> DSSDEASVSPIADNEREAVTLLLGYLEDKDQLDFYSGGPLKALTTLVYSDNLNLQRSAALAFAEITEKYVRQVSREVLEPILILLQSQDPQIQVAACAALGNLAVNNENKLLIVEMGGLEPLINQMMGDNVEVQCNAVGCITNLATRDDNKHKIATSGALIPLTKLAKSKHIRVQRNATGALLNMTHSEENRKELVNAGAVPVLVSLLSSTDPDVQYYCTTALSNIAVDEANRKKLAQTEPRLVSKLVSLMDSPSSRVKCQATLALRNLASDTSYQLEIVR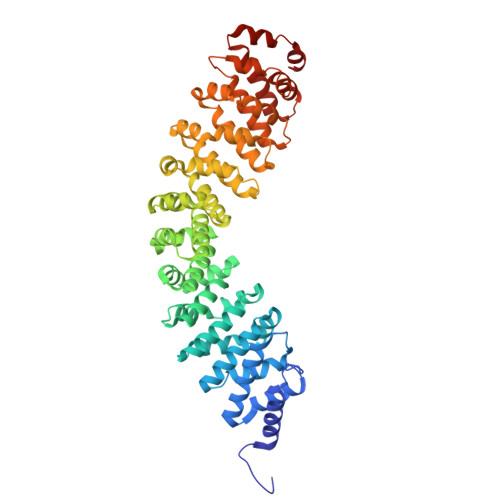AGGLPHLVKLIQSDSIPLVLASVACIRNISIHPLNEGLIVDAGFLKPLVRLLDYKDSEEIQCHAVSTLRNLAASSEKNRKEFFESGAVEKCKELALDSPVSVQSEISACFAILALADVSKLDLLEANILDALIPMTFSQNQEVSGNAAAALANLCSRVNNYTKIIEAWDRPNEGIRGFLIRFLKSDYATFEHIALWTILQLLESHNDKVEDLVKNDDDIINGVRK>MRGSHHHHHHGMASHMINKIFALPVIEQLTPVLSRRQLDDLDLIVVDHPQVKASFALQGAHLLSWKPVGEEEVLWLSNNTPFKTGVALRGGVPICWPWFGPAAQQGLPSHGFARNLPWALKAHNEDDNGVMLTFELQSSEATRKYWPHDFTLLARFKVGKTCEIELEAHGEFATTSALHSYFNVGDIANVKVSG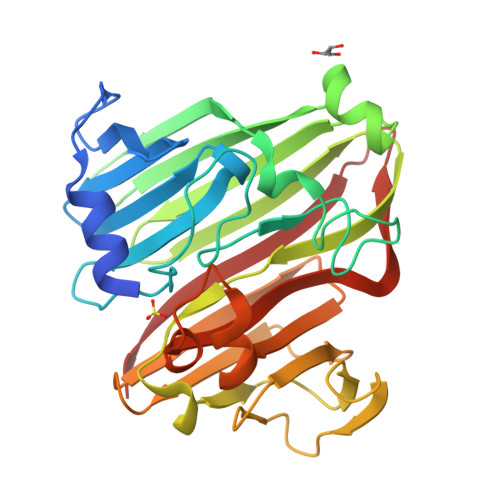LGDRFIDKVNDAKEGVLTDGIQTFPDRTDRVYLNPEACSVIHDATLNRTIDVVHHHHLNVVGWNPGPALSVSMGDMPDDGYKTFVCVETVYATAPQQATEEKPSRLAQTICVAKR[2x]N-METHYL-N-{2-[(2-NAPHTHYLSULFONYL)AMINO]-5-[(2-NAPHTHYLSULFONYL)OXY]BENZOYL}-L-ASPARTIC 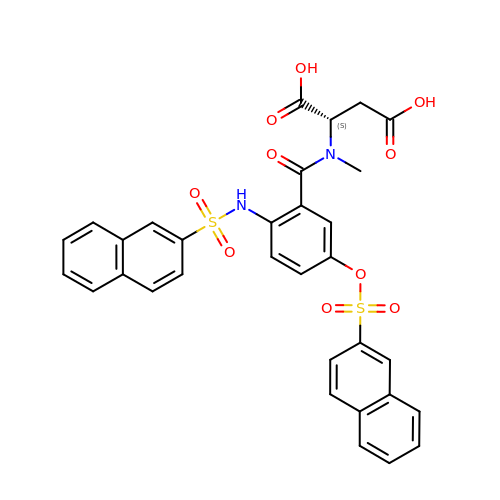ACID | C32 H26 N2 O10 S2 | JOAALZBSMWLOPQ-LJAQVGFWSA-N> GPMSSVQLSRGDFHSIFTNKQRYDNPTGGVYQVYNTRKSDGAN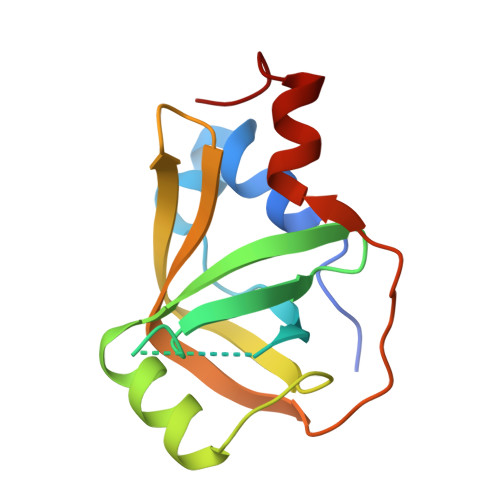SNRENLIMISDGIYHMKALLRNQAASKFQSMELQRGDIIRVIIAEPAIVRERKKYVLLVDDFELVQSRADMVNQTSTFLDNYFSEHPNETL> SVLSDFQEAVPTVVGIPDGTAVIGRSFRVSIPTDLIASSGEIIKVSAAGKEA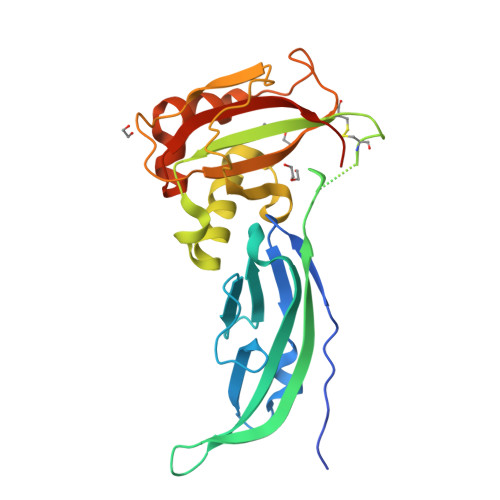LPSWLHWDPHSHILEGLPLDTDKGVHYISVSAARLGANGSHVPQTSSVFSIEVYPEDHNEPQSVRAASSDPGEVVPSACAADEPVTVLTVILDADLTKMTPKQRIDLLNRMQSFSEVELHNMKLVPVVNNRLFDMSAFMAGPGNAKKVVENGALLSWKLGCSLNQNSVPDIRGVETPAREGAMSAQLGYPVVGWHIANKKPTLPKRLRRQI> EESPFVGNPGNITGARGLTGTLRCQLQVQGEPPEVHWLRDGQILELADSTQTQVPLGEDEQDDWIVVSQLRITSLQLSDTGQYQCLVFLGHQTFVSQPGYVGLEGLPYFLEEPEDRTVAANTPFNLSCQAQGPPEPVDLLWLQDAVPLATAPGHGPQRSLHVPGLNKTSSFSCEAHNAKGVTTSRT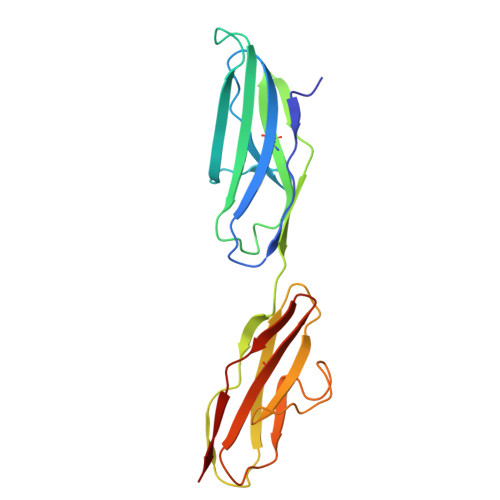ATITVLPQQ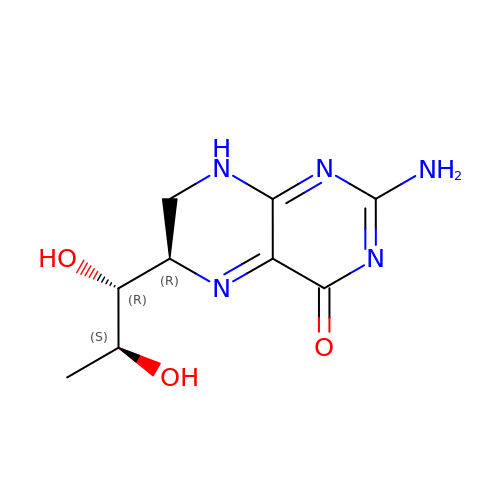2-AMINO-6-(1,2-DIHYDROXY-PROPYL)-7,8-DIHYDRO-6H-PTERIDIN-4-ONE | C9 H13 N5 O3 | ZHQJVZLJDXWFFX-RPDRRWSUSA-N> MKTKNRSNSIHASLRQLLALGLSKSSSAEPQRITRTVKFKINTDIRPDLIPVLNRHFDFFEKFRRKVLAELEALWNKDQKSFQAMVQCSAKKPYQKKTSCYAWLDTHFITEAKESLDLPRKPATSLLYNLSGGLKSFLTRRETVAEDIQKRFNDNLREWNGDLSQLASDLKAPLPPAPPNLDFENLIEKAIEKYNDWVGRTRAWCNLILVQQKKVERRDACLPRYLKGYPGFFGSQRYATTAGLAENLKKLEQVAREQSKKMPTRFAKLTPEIWTAIQERFSPPEVCEAGEKRRPRTAHQTVCLRFAALRAAHPEWTPVQLAEEILAGIFRGAEKLKKHLAANGFTDRPAVIKLANLYNVAAAFSLDPIRAAGDYILFYEEETPKRNAFGDVRGGLHQPSDESAAIEIMGFGLQKESGKPLYNGLLVCKKSEKEHDDSWAFLYCHTEGQTFELANEKAKLRGKLLTDWTGFASRGGSRKKAEASAKQLARGRVWISEKTPPTVLPLAFGSRQGREYLWHFDRDLREKNEWVLGNGRLLRIMPPGQPNAADFYLAITLERQVPPLADIKAERFIGIARGEAIPAAYAVIDELGKLLASGKIAESYRKQQREFNDAKRELQRTQGGYTRWLRSKERNRARALSGEVTRAVLALAAEHRAPVVLANLNSSLAMRGGKKTMMSLMQYQPVQRALE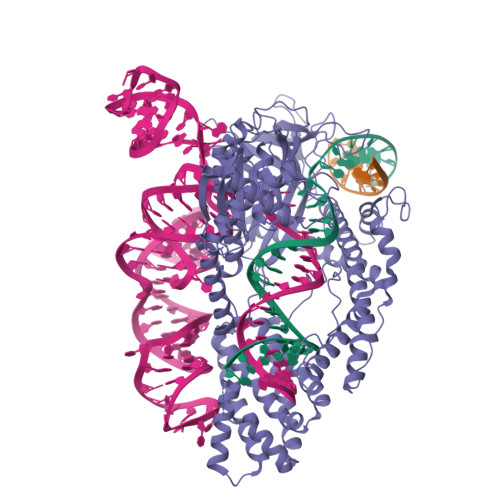QKFLEAGLWEAPKRKQKFPKKDNGFIKLIDAWWTSRTCSQCGNTHSSEFYEKLGETLTHAPDEKWCVTVCERPFVLPDTYQYRFRGEDKVGNTNERLQSLLKGKQIKELTGKQREHLIEFLERLLSFRPQQANFRCLKCGYETNAAVQAALTIARKYLFELEHPPKKGEKDRRLKWQAWYQEKLRTVWK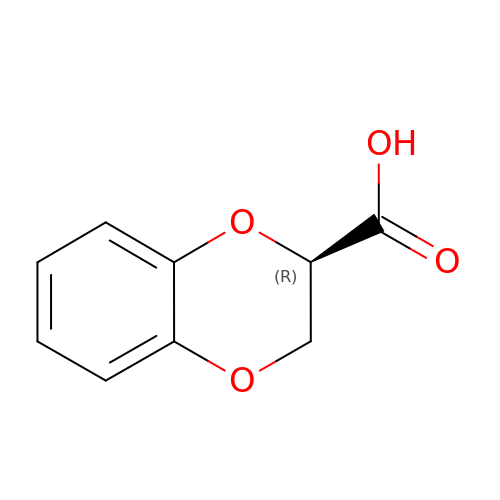(2R)-2,3-dihydro-1,4-benzodioxine-2-carboxylic acid | C9 H8 O4 | HMBHAQMOBKLWRX-MRVPVSSYSA-N> MTEYKIKATIEASVAKFKRQIDSAVKSVQRFKRVADQTKDVELNANDKKLQKTIKVAKKSLDAFSNKNVKAKLDASIQDLQQKILESNFELDKLNSKEASPEVKLQKQKLTKDIAEAENKLSELEKKRVNIDVNADNSKFNRVLKVSKASLEALNRSKAKAILDVDNSVANSKIKRTKEELKSIPNKTRSRLDVDTRLSIPTIYAFKKSLDALPNKKTTKVDVDTNGLKKVYAYIIKANDNFQRQMGNLANMFRVFGTVGSNMVGGLLTSSFSILIPVIASVVPVVFALLNAIKVLTGGVLALGGAVAIAGAGFVAFGAMAISAIKMLNDGTLQASSATNEYKKALDGVKSAWTDIIKQNQSAIFTTLANGLNTVKTAMQSLQPFFSGISRGMEEASQSVLKWAENSSVASRFFNMMNTTGVSVFNKLLSAAGGFGDGLVNVFTQLAPLFQWSADWLDRLGQSFSNWANSAAGENSITRFIEYTKTNLPIIGNIFKNVFAGINNLMNAFSGSSTGIFQSLEQMTAKFREWSEQVGQSQGFKDFVSYIQTNGPLIMQLIGNIARGLVAFATAMAPIASAVLRVAVAITGWIANLFEAHPATAQLVGVIITLVGAFRFLIAPILAVMDFLGPLAARLVALVTKFGWAKTGTLVLSKAMTSLKGPIKLVTAIFQLLFGKIGLIRNAITGLVTVFGILGGPITIVIGVIAALIAIFVLLWNKNEGFRNFIINAWNAIKTFMVNVWNVLKAVASVVWNAILTAITTAVSN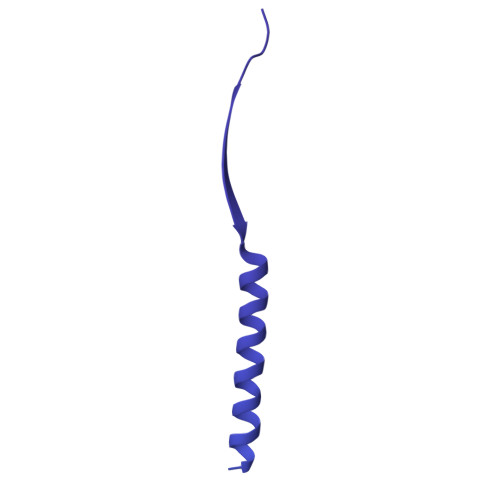VYNFIMIVWNQIVAYLQGLWNGIIAIATTVWNLLVTIITTVFTTIMTIVMTIWTAIWTFLSTIWNTIITIATTIWNLLVTVITTVFTTIMTIAMTIWNAIWTFLQTLWNTIVTVATKVWNAITTAISTALQAAWSFISNIWNTIWSFLSGILTTIWNKVVSIFTQVVSTISDKMSQAWNFIVTKGMQWVSTITSTLINFVNRVIQGFVNVVNKVSQGMTNAVNKIKSFIGDFVSAGADMIRGLIRGIGQMAGQLVDAAKNVAKKALDAAKSALGIHSPSREFMDVGMYSMLGFVKGIDNHSSKVIRNVSNVADKVVDAFQPTLNAPDISSITGNLSNLGGNINAQVQHTHSIETSPNMKTVKVEFDVNNDALTSIVNGRNAKRNSEYYL> GTVPPFIQPFEFPRFSIGQRVFIPCVVVSGDLPITITWQKDGRPIPGSLGVTIDNIDFTSSLRISNLSLMHNGNYTCIARNEAAAVEHQSQLIVRVPPKFVVQPRDQDGIYGKAVILNCSAEGYPVPTIVWKFSKGAGVPQFQPIALNG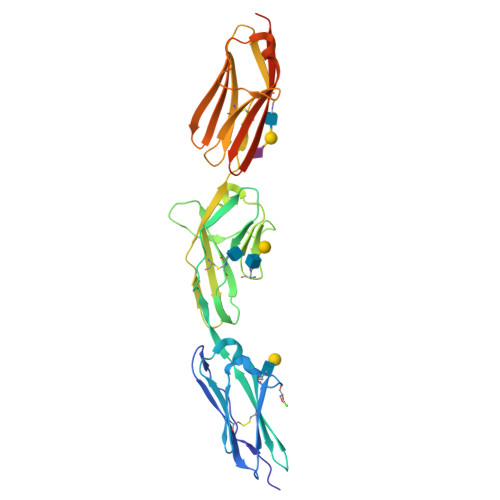RIQVLSNGSLLIKHVVEEDSGYYLCKVSNDVGADVSKSMYLTVKIPAMITSYPNTTLATQGQKKEMSCTAHGEKPIIVRWEKEDRIINPEMARYLVSTKEVGEEVISTLQILPTVREDSGFFSCHAINSYGEDRGIIQLTVQEELENLYFQGSHHHHHH>[2x]GADDELYRQ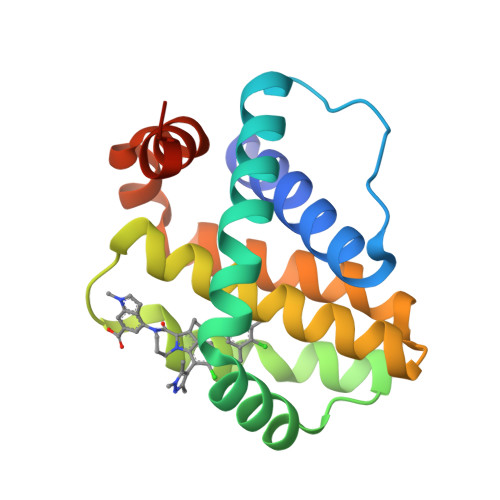SLEIISRYLREQATGAKDTKPMGRSGATSRKALETLRRVGDGVQRNHETAFQGMLRKLDIKNEDDVKSLSRVMIHVFSDGVTNWGRIVTLISFGAFVAKHLKTINQESCIEPLAESITDVLVRTKRDWLVKQRGWDGFVEFFHVEDLEGG> SYRDK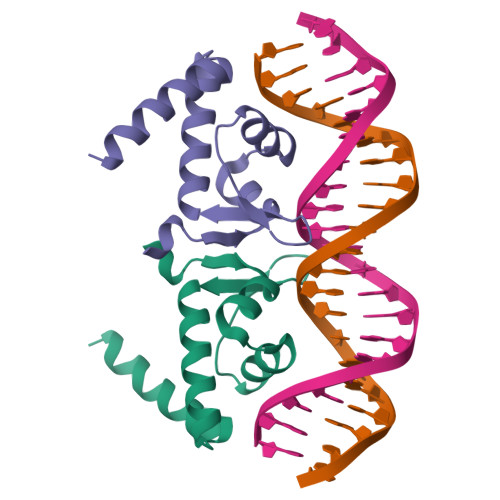KVMSIGIVKELTGLSERQIRYYEKRSLLFPDRTNTGIRKYSFSDVERLMDIADRIEEGVQTSEIRTELAKKDEARKM>[9x]MLGSLVLRRKALAPRLLLRLLRSPTLRGHGGASGRNVTTGSLGEPQWLRVATGGRPGTSPALFSGRGAATGGRQGGRFDTKCLAAATWGRLPGPEETLPGQDSWNGVPSRAGLGMCALAAALVVHCYSKSPSNKDAALLEAARANNMQEVSRLLSEGADVNAKHRLGWTALMVAAINRNNSVVQVLLAAGADPNLGDDFSSVYKTAKEQGIHSLEVLITREDDFNNRLNNRASFKGCTALHYAVLADDYRTVKELLDGGANPLQRNEMGHTPLDYAREGEVMKLLRTSEAKYQEKQRKREAEERRRFPLEQRLKEHIIGQESAIATVGAAIRRKENGWYDEEHPLVFLFLGSSGIGKTELAKQTAKYMHKDAKKGFIRLDMSEFQERHEVAKFIGSPPGYVGHEEGGQLTKKLKQCPNAVVLFDQVDKAHPDVLTIMLQLFDEGRLTDGKGKTIDCKDAIFIMTSNVASDEIAQHALQLRQEALEMSRNRIAENLGDVQISDKITISKNFKENVIRPILKAHFRRDEFLGRINEIVYFLPFCHSELIQLVNKELNFWAKRAKQRHNITLLWDREVADVLVDGYNVHYGARSIKHEVERRVVNQLAAAYEQDLLPGGCTLRITVEDSDKQLLKSPELPSPQAEKRLPKLRLEIIDKDSKTRRLDIRAPLHPEKVCNTI

The human AAA+ ATPase CLPB (SKD3) is a protein disaggregase in the mitochondrial intermembrane space (IMS) and functions to promote the solubilization of various mitochondrial proteins. Unlike canonical AAA+ proteins, CLPB contains a unique ankyrin repeat domain (ANK) at its N-terminus. The N-terminus of CLPB has a mitochondrial targeting signal (MTS), followed by an ankyrin repeat (ANK) domain, and ends with a C-terminal NBD. The ANK domain is not only responsible for maintaining the higher-order assembly but also essential for the disaggregase activity.

Two mutant versions of CLPB (NBD and NBDE425Q) were analyzed by cryo-EM, which again confirmed that E425Q mutation resulted in co-purification of an endogenous peptide in the central channel. After several rounds of 3D classification, 3 different oligomeric arrangements, hexameric, heptameric, and nonameric, were identified. The nonamer appeared to be more stable and could be resolved at an overall resolution of 3.7 Å, allowing the atomic modeling of the NBD of CLPB. In the nucleotide-binding pockets of the nonamer, a total of 8 ATP molecules could be modeled. The conserved residues I317, I318, and F541 form a hydrophobic pocket to stabilize the adenine ring of ATP, while T358 stabilizes the β- and γ-phosphates through a Mg2+ ion. In the nonamer, 9 protomers form a 1.5-turn helix around the central substrate. The density of the polypeptide backbone is well resolved in the nonamer and was modeled as a 17-residue poly-alanine fragment. For each protomer, a canonical PL-I (399-GYVG-402) binds to the peptide through 2 hydrogen bonds formed between the main-chain atoms. The first is between the carbonyl oxygen of the substrate residue N and the main-chain nitrogen of V401, and the other between the carbonyl oxygen of G399 and the main-chain nitrogen of the substrate residue N+2. Thus, the axial step size of PLs is exactly 2 residues.>[2x]HHHHHHSSGLVPRGSMTTDTHTLHIEEILDLLPHRFPFLLVDRVLDFEEGKFLRAVKNVSFNEPFFQGHFPGKPIF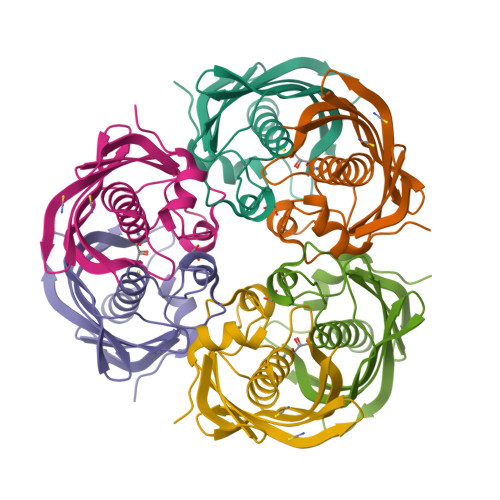PGVLILEAMAQATGILAFKSRGKLEPGELYYFAGIDEARFKRPVVPGDQMIMEVEFVKERRGLTRFTGVAKVDGEIVCTATMMCARSKPAAPAESVVVKPDVVKPDVVKPDVVNPVVKES> LMTVSKFASICTMGAN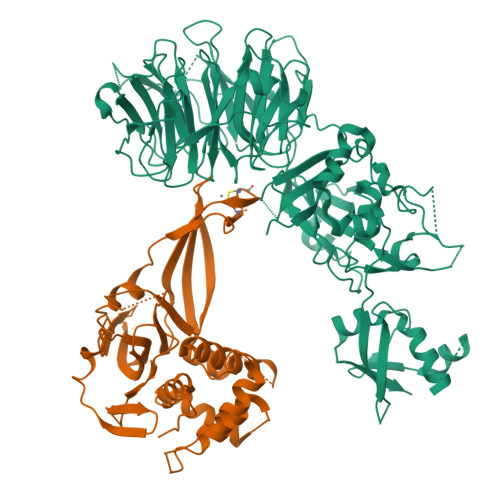ASALEKEIGPEQFPVNEHYFGLVNFGNTCYCNSVLQALYFCRPFREKVLAYKSQPRKKESLLTCLADLFHSIATQKKKVGVIPPKKFITRLRKENELFDNYMQQDAHEFLNYLLNTIADILQEERKQEKQNGRLPNGNIDNENNNSTPDPTWVHEIFQGTLTNETRCLTCETISSKDEDFLDLSVDVEQNTSITHCLRGFSNTETLCSEYKYYCEECRSKQEAHKRMKVKKLPMILALHLKRFKYMDQLHRYTKLSYRVVFPLELRLFNTSGDATNPDRMYDLVAVVVHCGSGPNRGHYIAIVKSHDFWLLFDDDIVEKIDAQAIEEFYGLTSDISKNSESGYILFYQSRD;> MAAHHRQNTAGRRKVQVSYVIRDEVEKYNRNGVNALQLDPALNRLFTAGRDSIIRIWSVNQHKQDPYIASMEHHTDWVNDIVLCCNGKTLISASSDTTVKVWNAHKGFCMSTLRTHKDYVKALAYAKDKELVASAGLDRQIFLWDVNTLTALTASNNTVTTSSLSGNKDSIYSLAMNQLGTIIVSGSTEKVLRVWDPRTCAKLMKLKGHTDNVKALLLNRDGTQCLSGSSDGTIRLWSLGQQRCIATYRVHDEGVWALQVNDAFTHVYSGGRDRKIYCTDLRNPDIRVLICEEKAPVLKMELDRSADPPPAIWVATTKSTVNKWTLKGIHNFRASGDYDNDCTNPITPLCTQPDQVIKGGASIIQCHILNDKRHILTKDTNNNVAYWDVLKACKVEDLGKVDFEDEIKKRFKMVYVPNWFSVDLKTGMLTITLDESDCFAAWVSAKDAGFSSPDGSDPKLNLGGLLLQALLEYWPRTHVNPMDEEENEVNHVNGEQENRVQKGNGYFQVPPHTPVIFGEAGGRTLFRLLCRDSGGETESMLLNETVPQWVIDITVDKNMPKFNKIPFYLQPHASSGAKTLKKDRLSASDMLQVRKVMEHVYEKIINLDNESQTTSSSNNEKPGEQEKEEDIAVLAEEKIELLCQDQVLDPNMDLRTVKHFIWKSGGDLTLHYRQKST> KTYRRSYTHAKPPYSYISLITMAIQQSPNKML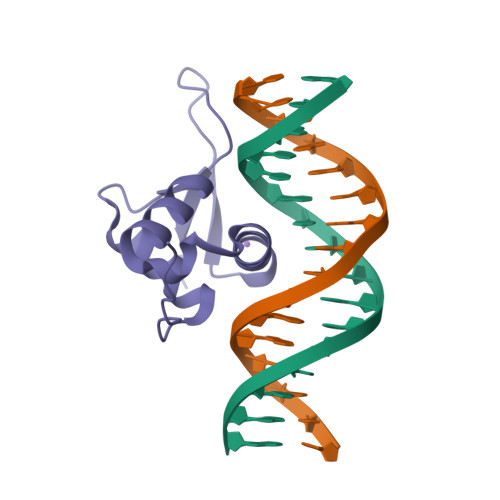TLSEIYQWIMDLFPFYRQNQQRWQNSIRHSLSFNDCFLKVPRSPDKPGKGSFWTLHPDSGNMFENGCYLRRQKRFKCEKQLALKEAAGAAGSG>[4x]AKHQERVQRLKEECEAGSRELKRCKEE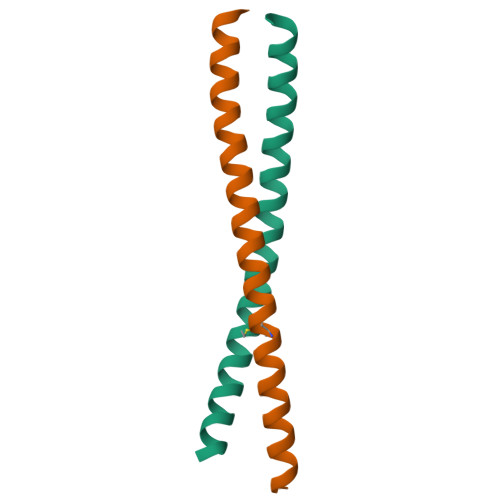NYDLAMRLAHQSEEKGAALMRNRDLQLEIDQLK2'-DEOXY-5'-O-[(S)-HYDROXY(PHOSPHONOMETHYL)PHOSPHORYL]URIDINE | 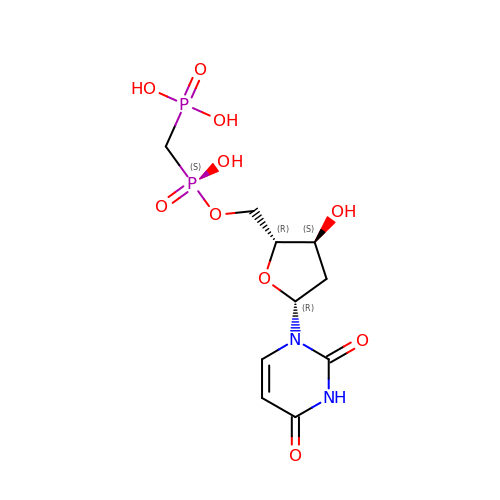C10 H16 N2 O10 P2 | MYBNSHXDOWMNJH-LKEWCRSYSA-N>[4x]SNAMNSILSLIGRDTELFHQDINANEKELQSVVSQSRFLVLGGAGSIGQAVTKEIFKRNPQKLHVVDISENNMVELVRDIRSSFGYINGDFQTFALDIGSIEYDAFIKADGQYDYVLNLSALKHVRSEKDPFTLMRMIDVNVFNTDKTIQQSIDAGAKKYFCVSTDKAANPVNMMGASKRIMEMFLMRKSEEIAISTARFANVAFSDGSLLHGFNQR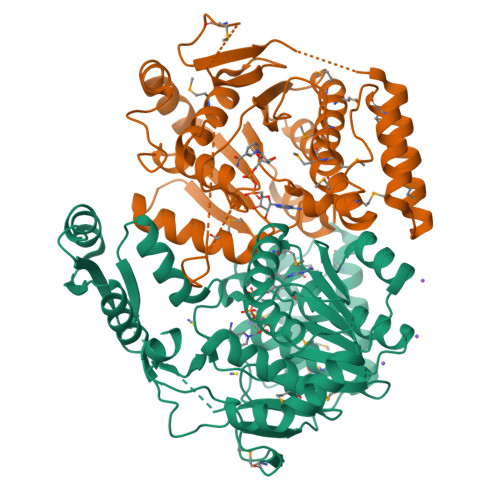IQKNQPIVAPNDIKRYFVTPQESGELCLMSCIFGENRDIFFPKLSEALHLISFADIAVKYLKQLGYEPHLCESEDEARELAKTLPAQGKWPCLFTSSDTTGEKDFEEFFTDKETLDMARFDNLGIIKNDSLYQQELLELFEQKIGQMKTDRQWTKEEIVQLFFIMIPDFGHKETGKYLDSKM2-(methylamino)ethyl dihydrogen 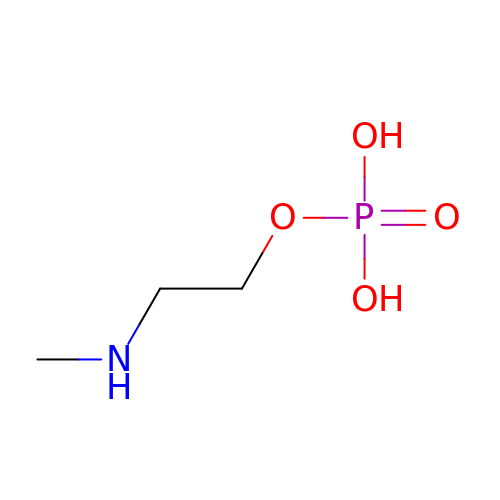phosphate | C3 H10 N O4 P | HZDCAHRLLXEQFY-UHFFFAOYSA-N>[2x]SVP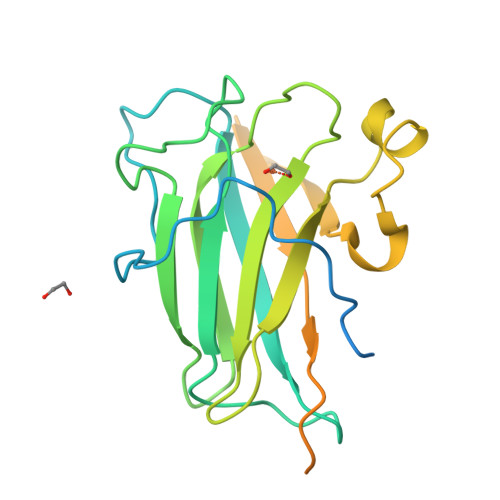LVAGGGAALARDTGAGAVPLAPTPACDDGDDPTPDQMEGPYFKPDSPPRTSLVTSSTPGVPLTVSGYVFGRACKPLTGVLLDFWQADTGGAYDMTGFAFRGHQFTGADGSFTLRTIVPGLYPGRTRHIHVKAQAPGRPVLTTQLYFPGEPRNTTDALFDPALLMNVRSAGPGREGTFDFVLDVAQQPDPTDPPTDPPGGGGWAAGTTYRAGDRVTYGGGSYRCLQAHTAVAGWEPPLVPALWERG> FKDPNAPKRPPSAFFLFCSEYRPKIKGEHPGLSIGDVAKKLGEMWNNTAADDKQPYEKKAAKLKEKYEKDIAAYR;> AQNITARIGEPLVLKCKGAPKKPPQRLEWKLNTGRTEAWKVLSPQGGGPWDSVARVLPNGSLFLPAVGIQDEGIFRCQAMNRNGKETKSNYRVRVYQIPGKPEIVDSASELTAGVPNKVGTCVSEGSYPAGTLSWHLDGKPLVPNEKGVSVKEQTRRHPETGLF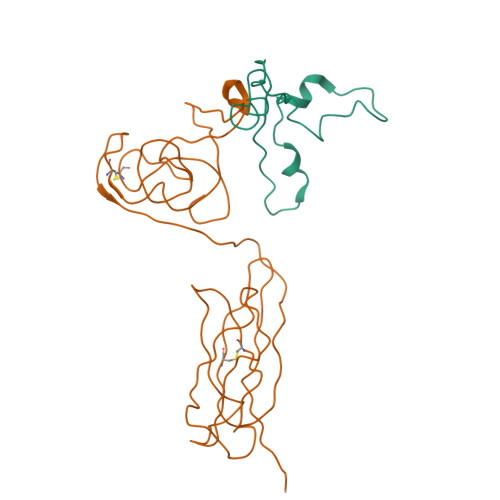TLQSELMVTPARGGDPRPTFSCSFSPGLPRHRALRTAPIQPRVWEPV>[2x]KIIVK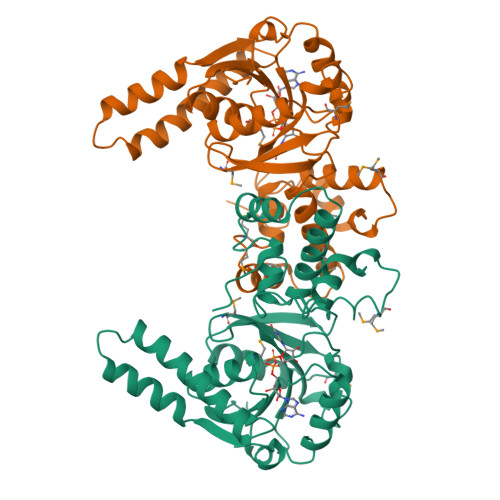HVTVIGGGLMGAGIAQVAAATGHTVVLVDQTEDILAKSKKGIEESLRKVAKKKFAENPKAGDEFVAKTLSTIATSTDAASVVHSTDLVVEAIVENLKVKNELFKRLDKRAAEHTIFASNTSSLQITSIANATTRQDRFAGLHFFNPVPVMKLVEVIKTPMTSQKTFESLVDFSKALGKHPVSCKDTPGFIVNRLLVPYLMEAIRLYERGDASKEDIDTAMKLGAGYPMGPFELLDYVGLDTTKFIVDGWHEMDAENPLHQPSPSLNKLVAENKFGKKTGEGFYKYKAA>GSAEALNNLGNVYRKQGDYQKAIEYYQKALELDPNNAEALNNLGNVYRKQGDYQKAIEYYQKALELDPNNAEALNNLGNVYRKQGDYQKAIEYYQKALELDPNNAEALNNLGNVYRKQGDYQKAIEYYQKALELDPNNAEALNNLGNVQRKQG[2x]

Here, we use single-molecule optical tweezers to study the folding of consensus-designed tetratricopeptide repeats (CTPRs), superhelical arrays of short helix-turn-helix motifs. The packing of the TPR motif results in superhelical structures, which means that, of all the different repeat-protein types, TPR arrays most closely resemble a physical spring. The starting point for this study was a consensus-designed TPR protein (referred to as CTPRa) that adopts a superhelical structure within the crystal lattice. This superhelical geometry of the TPRs is established through stacking of the A-helix (Ai+1 in Figure 1A) of a given repeat against both A- and B-helices of the preceding repeat (Ai and Bi in Figure 1A). The resulting angles between repeat planes then give rise to the pitch and diameter of the superhelix.

We used X-ray crystallography to determine the structure of a construct composed of 4 repeats of the new variant and a C-terminal solvating helix, CTPRrv4, to 3.0 Å resolution. CTPRrv4 crystallized in the P3121 space group with two molecules per asymmetric unit. As was observed for CTPRa, the C-terminal solvating helix was not resolved due to a higher preference for end-to-end stacking between molecules in neighboring asymmetric units. The resolution was sufficient to determine the change in repeat plane angles using the Cα coordinates: while the twist remained almost unchanged, an increase in the curvature is compensated by a similar decrease in bending. Although these changes may at first appear insignificant in the context of a 4-repeat array, they translate into clear differences in the longer superhelical arrays, leading to a decrease in helix length and increase in helix diameter. Furthermore, when compared to other CTPRs, all of which exhibit backbone RMSDs within 0.72 Å, the CTPRrv backbone differs by 1.4 Å relative to the CTPRa backbone. Circular dichroism spectroscopy of the 5-repeat proteins used in this study shows that the CTPR α-helicity remains intact in the new repeat type. Whereas CTPRa variants unfolded and refolded at a plateau force of ≈12.5 pN, the plateau of CRPRrv was significantly lower at ≈9.5 pN, indicating that the introduced mutations have a destabilizing effect. Importantly, the overall lower stability of the rv-type arrays relative to CTPRa arrays is due to a larger destabilization of the intrinsic energy than the destabilization of the interfacial energy (ΔΔGunit ≈ 3 kBT and ΔΔGnn ≈ 1.7 kBT, respectively). On the contrary, a single CTPRrv repeat is unstable (1.1 ± 0.2 kBT) and requires the energy from the interface with at least one more helix to fold.> ADPQAGSLDLQIDEEQPAGTLIGDISAGLPAGTAAPLMYFISAQEGSGVGTDLAIDEHSGVVRTARVLDREQRDRYRFTAVTPDGATVEVTVRVADINDHAPAFPQARAALQVPEHTAFGTRYPLEPARDADAGRLGTQGYALSGDGAGETFRLETRPGPDGTPVPELVVTGELDRENRSHYMLQLEAYDGGSPPRRAQALLDVTLLDINDHAPAFNQSRYHAVVSESLAPGSPVLQVFASDADAGVNGAVTYEINRRQSEGDGPFSIDAHTGLLQLERPLDFEQRRVHELVVQARDGGAHPELGSAFVTVHVRDAN;> MDLAPDRATGRPWLPLHTLSVSQLLRVFWLLSLLPGQAWVHGAEPRQVFQVLEEQPPGTLVGTIQTRPGFTYRLSESHALFAINSSTGALYTTSTIDRESLPSDVINLVVLSSAPTYPTEVRVLVRDLNDNAPVFPDPSIVVTFKEDSSSGRQVILDTATDSDIGSNGVDHRSYRIIRGNEAGRFRLDITLNPSGEGAFLHLVSKGGLDREVTPQYQLLVEVEDKGEPKRRGYLQVNVTVQDINDNPPVFGSSHYQAGVPEDAVVGSSVLQVAAADADEGTNADIRYRLQDEGTPFQMDPETGLITVREPLDFEARRQYSLTVQAMDRGVPSLTGRAEALIQLLDVNDNDPVVKFRYFPATSRYASVDENAQVGTVVALLTVTDADSPAANGNISVQILGGNEQRHFEVQSSKVPNLSLIKVASALDRERIPSYNLTVSVSDNYGAPPGAAVQARSSVASLVIFVND

The atypical cadherins Fat and Dachsous are key regulators of cell growth and animal development. In contrast to classical cadherins, which form homophilic interactions to segregate cells, Fat and Dachsous cadherins form heterophilic interactions to induce cell polarity within tissues. Here, we determine the co-crystal structure of the human homologs Fat4 and Dachsous1 (Dchs1) to establish the molecular basis for Fat-Dachsous interactions. Fat4 and Dchs1 are two of the largest members of the cadherin superfamily and contain 34 and 27 extracellular cadherin (EC) domains, respectively.

The Fat4(EC4):Dchs1(EC1) interface contains a hydrophobic cluster centered on Leu379 of Fat4(EC4) and Val120 of Dchs1(EC1). Within this cluster, Fat4 contributes a majority of hydrophobic residues including Val376, Leu417, and Leu419, which contact the methyl groups of Thr118 and Thr126 of Dchs1. On the Dchs1 side, the main contacts are formed by the sidechain of Phe79 and the main chain of β-strand 3. Additional backbone hydrogen bonding interactions can be seen flanking the hydrophobic cluster between the amine of Val376 and the carbonyl of Pro122, between Thr383 and the amine of Glu84, from the epsilon nitrogen of Arg356 to the carbonyl of I80, and from Gln83 to the carbonyl of Val382. The EC2:EC3 interfaces are largely hydrophilic and are formed between the β6 and β7 strands of the respective EC3 domains. A small hydrophobic core can be found in the Fat4(EC2):Dchs1(EC3) interface containing anchors Fat4-Phe199 and Dchs1-Phe347, in addition to Fat4-Ile155 and Dchs1-Val331. Extensive hydrogen bond networks can be found centered around Arg297 in the β3–β4 loop of Dchs1(EC3) and Asn152 located in the β4–β5 loop of Fat4(EC2). By contrast the Fat4(EC3):Dchs1(EC2) interface is devoid of any close contacts. The alignment of EC2–EC3 of each protein revealed that the EC1 of Dchs1 is tilted by ~35° towards Fat4, making it the only protomer that adopts such a pronounced curvature in a protocadherin-like binding interface. This distinctive conformation was observed in both the high- and low-resolution structures.>[2x]MGSKRRFSSEHPDPVETSIPEQAAEIAEELSKQHPLPSEEPLVHHD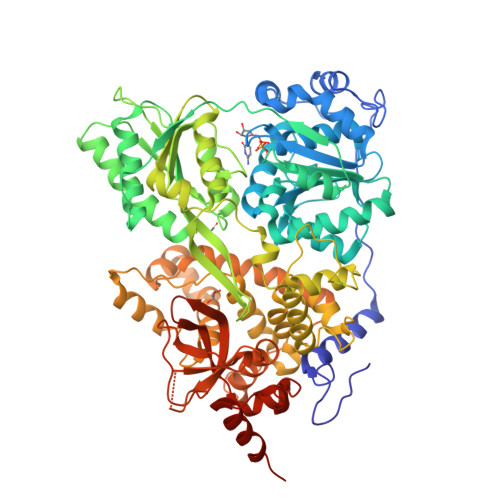AGEFKGLQRHHTSAEEAQKLEDGKINPFTGREFTPKYVDILKIRRELPVHAQRDEFLKLYQNNQIMVFVGETGSGKTTQIPQFVLFDEMPHLENTQVACTQPRRVAAMSVAQRVAEEMDVKLGEEVGYSIRFENKTSNKTILKYMTDGMLLREAMEDHDLSRYSCIILDEAHERTLATDILMGLLKQVVKRRPDLKIIIMSATLDAEKFQRYFNDAPLLAVPGRTYPVELYYTPEFQRDYLDSAIRTVLQIHATEEAGDILLFLTGEDEIEDAVRKISLEGDQLVREEGCGPLSVYPLYGSLPPHQQQRIFEPAPESHNGRPGRKVVISTNIAETSLTIDGIVYVVDPGFSKQKVYNPRIRVESLLVSPISKASAQQRAGRAGRTRPGKCFRLYTEEAFQKELIEQSYPEILRSNLSSTVLELKKLGIDDLVHFDFMDPPAPETMMRALEELNYLACLDDEGNLTPLGRLASQFPLDPMLAVMLIGSFEFQCSQEILTIVAMLSVPNVFIRPTKDKKRADDAKNIFAHPDGDHITLLNVYHAFKSDEAYEYGIHKWCRDHYLNYRSLSAADNIRSQLERLMNRYNLELNTTDYESPKYFDNIRKALASGFFMQVAKKRSGAKGYITVKDNQDVLIHPSTVLGHDAEWVIYNEFVLTSKNYIRTVTSVRPEWLIEIAPAYYDLSNFQKGDVKLSLERIKEKVDRLNELKQGKNKKKSKHSKK>MHHHHHHKNITNASILSIVYKDDDLIDLSRYGAEIYNGDKVYYNSIDKNQIRLINLESSTIEVILKKAIVYNSMYENFSTSFWIRIPKYFNSISLNNEYTIINCMENNSGWKVSLNYGEIIWTFQDTQEIKQRVVFKYSQMINISDYINRWIFVTITNNRITKSKIYINGRLIDQKPISNLGNIHASNKIMFKLDGCRDPHRYIVIKYFNLFDKELSEKEIKDLYDNQSNSGILKDFWGDYLQYDKSYYMLNLYDPNKYVDVNNVGIRGYMYLKGPRDNVMTTNIYLNSSLYMGTKF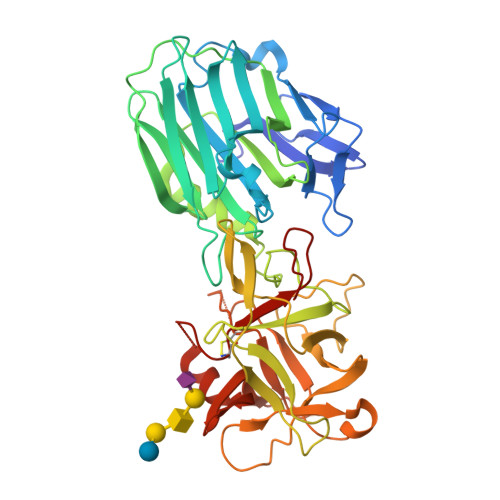IIKKYASGNKDNIVRNNDRVYINVVVKNKEYRLATNASQAGVEKILSALEIPDVGNLSQVVVMKSKNDQGITNKCKMNLQDNNGNDIGFIGFHQFNNIAKLVASNWYNRQIERSSRTLGCSWEFIPVDDGWRERPL[2x]In the present study, we prepared a marine invertebrate ferritin from Dendrorhynchus zhejiangensis (DzFer) and found that it could withstand extreme pH fluctuation. The majority of ferritins consist of 24 subunits assembled in a highly symmetric manner. They compose a spherical protein shell around a central cavity into which a ferric oxyhydroxide mineral core can be formed. As is well known, these subunits are reversibly assembled into a hollow nanocage with a diameter of ~12 nm and a 4-3-2 symmetrical architecture, resulting in six four-fold, eight three-fold and twelve two-fold channels.

For the soaking method, DzFer crystals grown from condition I were soaked for 1 min in the condition I solution supplemented with 20% glycerol and 100 mM AgNO3. On the basis of the X-ray crystallographic analysis, the refined structure of Ag+-DzFer showed that a total of 88 Ag+ ions were bound to the DzFer nanocage through metal-coordination bonds. The fold of one subunit in Ag+-DzFer was composed of an antiparallel four-helix bundle together with a tiny helix E located at the end of the DE loop, where five Ag+-binding sites were observed near the helix A, the BC loop, and the CD loop. Notably, the ferroxidase site was assigned one Ag+ ion because putting the Fe3+ here could produce a prominent negative Fo–Fc electron density map. In the Ag+ cocrystal structure of DzFer, two Ag+-binding sites (Ag1 and Ag2) were observed inside the three-fold channel, whereas the other three Ag+-binding sites (Ag3, Ag4, and Ag5) were observed at the outer surface groove of the Ag+-DzFer shell through metal-coordination bonds. Ag1 was ligated by the carboxylate groups of Glu130 residues at distances of 2.7 Å and three water molecules at distances of 2.3 Å. Ag2 was coordinated with the carboxylate groups of the Asp127 (at distances of 3.2 Å) and Glu130 (at distances of 2.9 Å) residues and three water molecules (at distances of 3.3 Å). In the Ag+-DzFer structure, although few studies regarding ferritin with structural data to support this, we observed an argentophilic interaction between Ag1 and Ag2 (the Ag-Ag distance of 2.5 Å), and they coordinated with the negatively charged residues Asp127 and Glu130 at the three-fold channel. Ag4 was ligated by the thiolate group of the Cys12 residue at a distance of 3.1 Å, the carboxylate group of the Asp122 residue at a distance of 2.7 Å, and one water molecule at a distance of 2.7 Å. At the site of Ag5, the Ag+ ion was coordinated with the thioether group of Met31 at a distance of 3.2 Å, the hydroxyl group of Ser35 at a distance of 3.8 Å, and one water molecule at a distance of 2.7 Å.

> MSLCRQNYHEECEAGVNKQINMEFYASYVYMSMASHFDRDDVALKGAHEFFLKSSSEEREHAMRLIKFQNQRGGRVVYQDIKKPEKDAWGTLTDAMQAALDLEKHVNQALLDLHALASKHNDPQMCDFIENHYLTEQVEAIREISGYLTNLKRCGPGLGEFLFDKELNS>[6x]MRGSHHHHHHGSMDKNIIIGAMTALITPFKNGKVDEQSYARLIKRQIENGIDAVVPVGTTGESATLTAEEHRTCIEIAVETCKGTKVKVLAGAGSNATHEAVGLAKFAKEHGADGILSVAPYYNKPTQQGLYEHYKAIAQSVDIPVLLYNVPGRT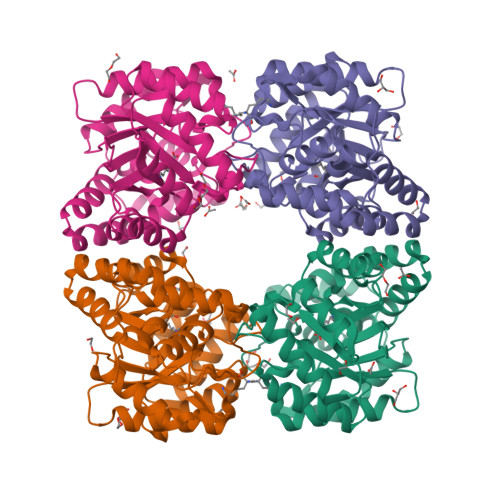GCEISTDTIIKLFRDCENIYGVKEASGNIDKCVDLLAHEPRMMLISGEDAINYPILSNGGKGVISVTSNLLPDMISALTHFALDENYKEAKKINDELYNINKILFCESNPIPIKTAMYLAGLIESLEFRLPLCSPSKENFAKIEEVMKKYKIKGF N-[oxo(pyridin-2-ylamino)acetyl]-beta-D-glucopyranosylamine | C13 H17 N3 O7 | 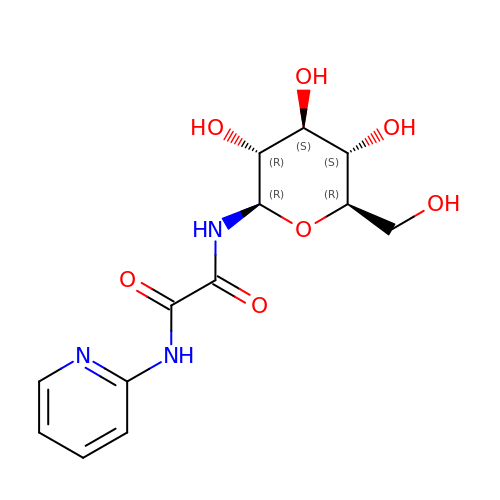XWDCGBAAIPNJDU-ODYQSLDMSA-N Contactins (CNTNs) are neural cell adhesion molecules that encode axon-target specificity during the patterning of the vertebrate visual and olfactory systems. Because CNTNs are tethered to the plasma membrane by a glycosylphosphatidylinositol anchor, they lack an intracellular region to communicate across the membrane. Instead, they form coreceptor complexes with distinct transmembrane proteins to transmit signals inside the cell. Finally, structural analyses of five CNTN–amyloid pairs indicate that these proteins interact through a conserved interface involving the second fibronectin type III repeat of CNTNs and the copper-binding domain of amyloid proteins.

Because of the difficulty we encountered in obtaining the CNTN4–APPb crystals, we followed the strategy we employed for chicken CNTN3–APP crystals and generated a fusion protein between the FN1–FN2 region of zebrafish CNTN4 and the E1 domain of zebrafish APLP2. The structure of this chimeric protein was refined to 2.46 Å (Rwork/Rfree = 0.189/0.221). Overall, the CNTN4–APPb and CNTN4–APLP2 interfaces display many of the same features found in the cocrystals of chicken CNTN4 and APP. As is the case in previous CNTN–APP complex structures, the bulk of the interactions includes main chain–main chain hydrogen bonds between two β-strands: W751–Q753 in CNTN4 and L129–P132 in APPb or L134–P137 in APLP2. As is the case in the CNTN3–APP and CNTN4–APP interfaces, the carbonyl oxygen atom of S126 in APPb (S131 in APLP2) forms a hydrogen bond with the hydroxyl group of Y764. Furthermore, CNTN4 residues Y784 and E789 form hydrogen bonds with E141 and H139, respectively, in APPb, and with E146 and H144, respectively, in APLP2. Overall, the sum of this crystallographic work indicates that the CNTN4–APLP2 interface in zebrafish is essentially identical to the CNTN4–APPb interface in zebrafish and the CNTN4–APP interface in chicken. Finally, in APLP2, the alanine residue is replaced by a bulkier Cβ-branched valine, and the side chain of M752 appears to swing away from V133.

> GPGSPPGPPTSIHVEEITDTTATLSWRPGPDNHSPITAYTIQARTPFSLGWQAVSTVPEVVGGSHLTATVIELNPWVEYEFRVLASNAVGTGEPSKPSKKARTKDTVPKVTPANVSGGGGSRSELVITWEPVPEELQNGAGFGYVVAFRPFGSTGWMQAAVPSPEASKYVFKNETILPFSPFQVKVGAYNNKGEGPFGPVITIYSAEGGGSGGGSGYIEALAANAGTGFAVAEPQVAMFCGKLNMHINIQTGRWEPDPSGSKTCVGTKEGVLQYCQEIYPELQITNVVEANQPVKIENWCKKDKKQCKGHAHIVVPYKCLVGEFVSDVLLVPEKCKFFHKERMDMCVSHQQWHGVAKEACSKGNMVLHSYGMLLPCGIDKFHGTEYVCCPSTRPEEPAPPASPSKAAA>STLEIAGLVRKNLVQFGVGEKNGSVRWVMNALGVKDDWLLVPSHAYKFEKDYEMMEFYFNRGGTYYSISAGNVVIQSLDVGFQDVVLMKVPTIPKFRDITQHFIKKGDVPRALNRLATLVTTVN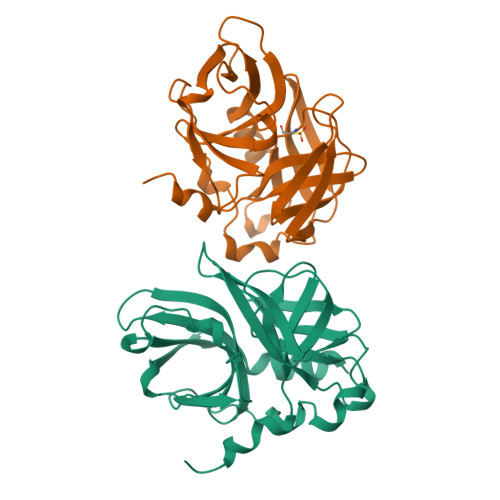GTPMLISEGPLKMEEKATYVHKKNDGTTVDLTVDQAWRGKGEGLPGMCGGALVSSNQSIQNAILGIHVAGGNSILVAKLVTQEMFQNIDKKIE[2x]> AKDGLG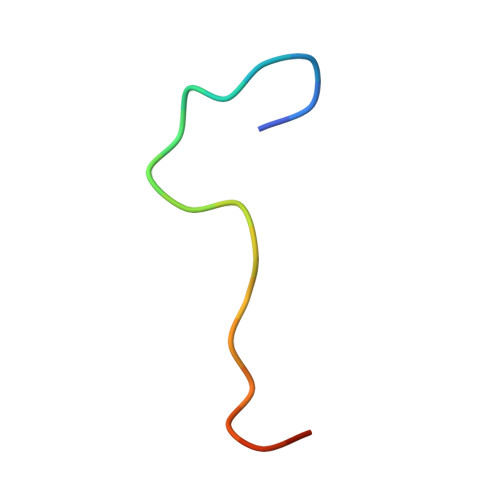EYTCTSLEGFEGK>QGHMAVRRVVANIATPEPARAQAFYGDILGMPVAMDHGWIVTHASPLEAHAQVSFAREGGSGTDVPDLSIEVDNFDEVHARILKAGLPIEYG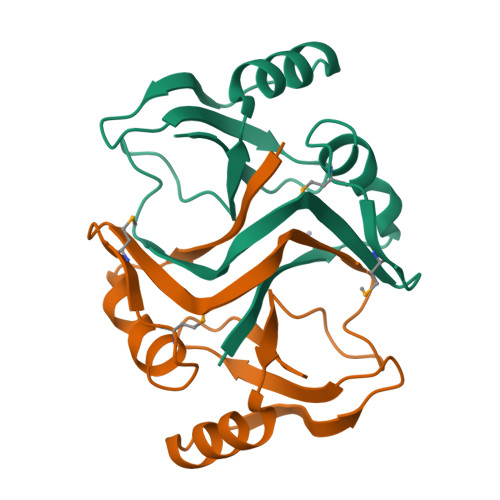PVTEAWGVQRLFLRDPFGKLINILSHA[2x]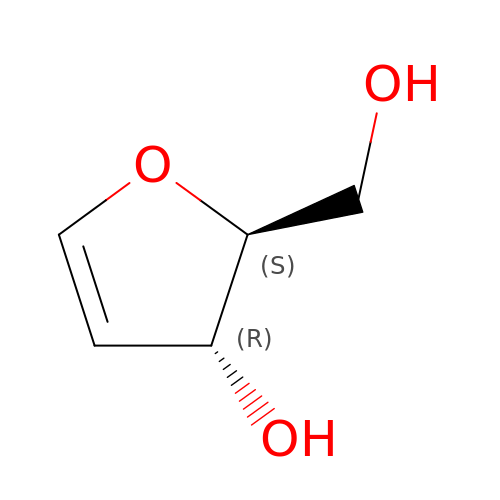2,5-anhydro-4-deoxy-D-erythro-pent-4-enitol | C5 H8 O3 | SGOSIWMWLVSBIC-UHNVWZDZSA-N> INIGNKTNENVISFFDSTDAETQNHNALMKGCGEFIVNLRTLLRTFRTITDNWILQANTKTPITDLTNTTDAQGRDYMSYLSYLYRFYRGGRRYKFFNTTPLKQSQTCYIRSFLIPRNYSADEINVDGPSHITYPVINPVHEVEVPFYSQYRKIPIASTSDKGYDSSLMYFSNTATTQIVARAGNDDFTFGWMIGPPQLQGESRSVAP;> NVHNTELASSTSENSVETQEITTFHDVETPNRIDTPMAQDTSSARNMDDTHSIIQFLQRPVLIDNIEIIAGTTADANKPLSRYVLDQQNSQKYVRSWTLPSTVLRAGGKAQKLANFKYLRCDVQVKLVLNANPFVAGRMYLAYSPYDDKVDTARSVLQTSRAGVTGYPGVELDFQLDNSVEMTIPYASFQEAYDLVTGTEDFVQLYLFPITPVLGPKSESESSKVDISVYMWLSNISLVIPTYRINP;> SKPRNQQQVCPLQNVPAWGYSLYKGIDMSVPLAYDPNNELGDLKDVFPSAVDEMAIGYVCGNPAVKHVLTWKTTDAIQKPIANGDDWGGVIPVGMPCYSKSIRTTRISATENRETEVMDAAPCEYVANMFSYWRATMCYRITVVKTAFHTGRLEIFFEPGVIPVKPTVNNIGPDQDRLTGAVAPSDNNYKYILDLTNDTEVTIRVPFVSNKMFLKTAGIYGANSENNWNFHESFSGFLCIRPVTKLMAPDTVSDNVSIVVWKWAEDVVVVEPKPLTSGPTQVYRPPPTASTAVEVLNVEL;> TSENPKIGPISEVASGVKTTANGIERIPVIGEIAKPVTTAVKWFADVVGTVAAIFGW

Israeli acute bee paralysis virus (IAPV) is a member of the Aparavirus genus of the family Dicistroviridae. Viruses of the family Dicistroviridae have nonenveloped icosahedral capsids protecting linear, single-stranded, positive-sense RNA genomes of 8,500 to 10,200 nucleotides. The major capsid proteins VP1 to VP3 of IAPV form the capsid shell with pseudo-T=3 icosahedral symmetry, whereas VP4 is a small protein attached to the inner surface of the capsid. Here we present a high-resolution cryo-EM analysis of IAPV virions induced to release their genomes in vitro.

The incubation of IAPV virions at 63°C resulted in a mixed population of full and empty particles. Cryo-EM images of the full particles were used to calculate a single-particle reconstruction to a resolution of 3.3 Å. The structure of the full virion could be built except for residues 1 to 10 and 258 to 318 of VP2. Residues 13 to 69 of VP4, among the 69 residues in the polypeptide, could be modeled in the cryo-EM map. The positioning of residue 69 from the C terminus of VP4 close to residues Asp186-Asp187-Phe188 of VP1 verifies the previous speculation that these residues form a putative catalytic site responsible for the cleavage of dicistrovirus VP0 into VP4 and VP3 subunits. The structure of the heated IAPV virion is nearly identical to that of the native virus, with a root mean square deviation (RMSD) of C-α atoms from the icosahedral asymmetric units of 0.76 Å. Accordingly, the internal volumes of the virion cavities are 6.2 × 106 Å3 and 6.3 × 106 Å3, respectively. This structural similarity indicates that IAPV does not form A particles before genome release. Whereas the capsid structures of the native and heated (63°C) IAPV virions were almost identical, there were differences in the distribution of the genomic RNA inside the particles. In heated IAPV virions, the RNA forms a 20-Å-thick shell with a higher density that tightly follows the inner face of the capsid and a sphere in the center of the virion with a radius of 80 Å. The changes in the distribution of RNA may facilitate the subsequent release of the genome from the IAPV virion.> MAGVKNSIIWFRKGLRLHDNPALLEACKDAKHVYPVFVLDPHFLQQSSYKVSVNRYNFLLESLEDLQRSFQARGSRLLVLRGKPEEVFPRVFREWGVTQLCFEHDTEPYAKVRDAAVRRLAAEAGVEVVTPISHTLYDTDMLVARNGGAAPLTMQSFTKLVDRVGDPPAPAPDPPAAMPPPAEDMPSAAPAATGVPTWQEVGFKEPPLTVFKGGETEALARLEAAFQDPKWVAGFQKPDTDPSAWEKPATTVLSPYLKFGCLSARLFHARLLEVYRRHPAHSQPPVSLRGQLLWREFFYTVGSTTPNFHRMAGNPVCKQIDWDDNPEFLAAWREARTGFPWIDAIMTQLVTWGWMHHLARHSVACFLTRGDLYVSWERGMEVFEEHLIDQDHYLNAANWMWLSASAFFSQYFRVYSPVVFGKKYDPEGRFIRKFLPVLKDMPAKYIYEPWTAPLEVQRKAGCVVGRDYPAPIVDHAVASKACIARMAAAYRRSKGEKLAAALEHHHHHH

Animal-like cryptochromes are photoreceptors that control circadian rhythm and signaling in many eukaryotes. As evolutionary transitional forms, some CRYs like the aCRY from Chlamydomonas reinhardtii (CraCRY) are bifunctional by acting both as photoreceptor and photolyase. CraCRY uses a tetrad of four aromatic residues (14–16) for FAD photoreduction and subsequent formation of the signaling-relevant FADH• state. Like in other PCSf members of the aCRY/(6–4) photolyase branch, these residues (CraCRY: W399, W376, W322, and Y373) form a 22-Å-long ET pathway from the surface of the C-terminal photolyase homology region (PHR) domain toward the FAD chromophore.

Without external reductant, FADox➔FADH• photoreduction of CraCRY stalls in the semiquinoid FADH• state. In CraCRY’s FADH• state, helix α22 (H475-K494) and two regions nearby, N314-D324 in the α13/α14 loop as well as A404-Q410 in the α18/α19 loop, are disordered because of lacking electron density. Consequently, the ET pathway along W399-W376-W322-Y373 to the FAD chromophore is broken. First, the Y373 side chain, which packs closely against W322 in FADox and FADH− states, is released from any interactions by becoming completely solvent exposed. Secondly, W322 is indispensable like Y373 for photoreduction but belongs now to the disordered α13/α14 loop. Moreover, the FADox➔FADH• transition causes loss of the prominent salt bridges between α22 and the PHR domain, namely D321-R485/R492, D323-R485 and D371-H475. The order-disorder transition upon FADH• state formation is unusual as a surface area of 870 Å2 from 14 α22 residues is occluded from solvent access by interacting with the PHR domain. CraCRY’s FADH• state structure provides numerous additional interaction sites for downstream signaling partners like the circadian clock factor ROC15 (33). Our in crystallo observation of a partly unfolded FADH• state prompts us to note that refolding to an FADox-like conformation, concomitant with restoration of the ET pathway from Y373 to the chromophore, is required for further FADH•➔FADH− photoreduction. In contrast, continuous illumination used to obtain the static FADH• state structure drives the reaction completely toward the signaling state.> GGCUUAUCAAGAGAGGGUGAGCGACUGGCGCGAAGAUCCCCGGCAACC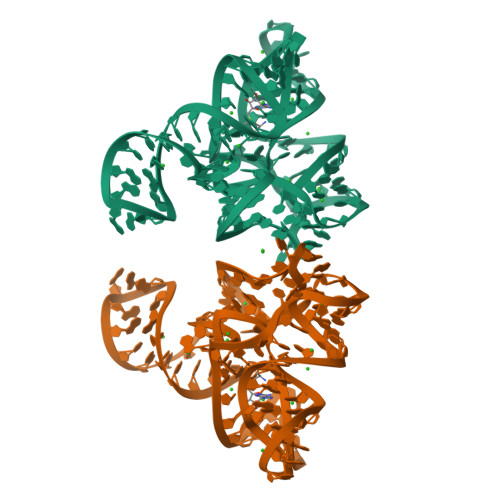AGAAAUGGUGCCAAUUCCUGCAGCGGAAACGUUGAAAGAUGAGCC> MFGSGNVLPVKIQPPLLRPLAYRVLSRKYGLSIKSDGLSALAEFVGTNIGANWRQGPATIKFLEQFAAVWKQQERGLFIDQSGVKEVIQEMKEREKVEWSHEHPIQHEENILGRTDDDENNSDDEMPIAADSSLQNVSLSSPMRQPTERDEYKQPFKPESSKALDWRDYFKVINASQQQRFSYNPHKMQFIFVPNKKQNGLGGIAGFLPDIEDKVQMFLTRYYLTNDRVMRNENFQNSDMFNPLSSMVSLQNELSNTNRQQQSSSMSITPIKNLLGRDAQNFLLLGLLNKNFKGNWSLEDPSGSVEIDISQTIPTQGHYYVPGCMVLVEGIYYSVGNK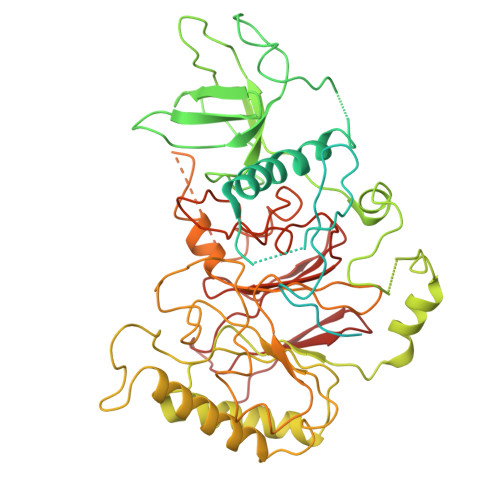FHVTSMTLPPGERREITLETIGNLDLLGIHGISNNNFIARLDKDLKIRLHLLEKELTDHKFVILGANLFLDDLKIMTALSKILQKLNDDPPTLLIWQGSFTSVPVFASMSSRNISSSTQFKNNFDALATLLSRFDNLTENTTMIFIPGPNDLWGSMVSLGASGTLPQDPIPSAFTKKINKVCKNVVWSSNPTRIAYLSQEIVIFRDDLSGRFKRHRLEFPFNESEDVYTENDNMMSKDTDIVPIDELVKEPDQLPQKVQETRKLVKTILDQGHLSPFLDSLRPISWDLDHTLTLCPIPSTMVLCDTTSAQFDLTYNGCKVINPGSFIHNRRARYMEYVPSSKKTIQEEIYI2-bromanyl-1-phenyl-ethanone | C8 H7 Br 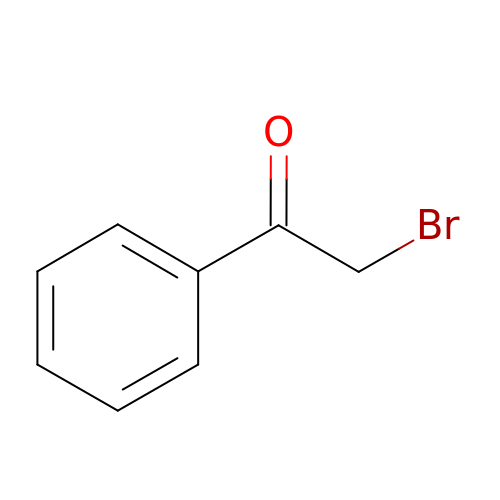O | LIGACIXOYTUXAW-UHFFFAOYSA-N>[2x]PKIVVVGAVAGGATCASQIRRLDKESDIIIFEKDRDMSFANCALPYVIGEVVEDRRYALAYTPEKFYDRKQITVKTYHEVIAINDERQTVSVLNRKTNEQFEESYDKLILSPGASANSLGFESDITFTLRNLEDTDAIDQFIKANQVDKVLVVGAGYVSLEVLENLYERGLHPTLIHRSDKINKLMDADMNQPILDELDKREIPYRLNEEINAINGNEITF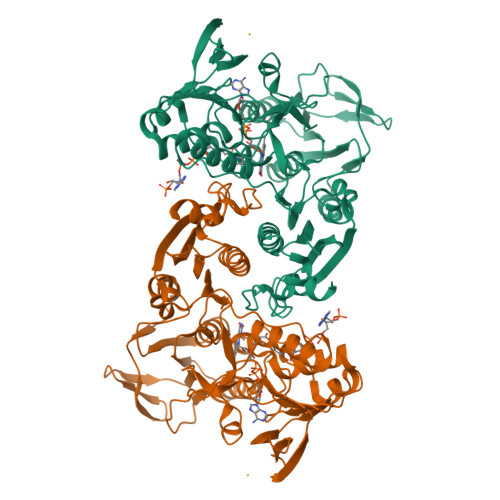KSGKVEHYDMIIEGVGTHPNSKFIESSNIKLDRKGFIPVNDKFETNVPNIYAIGDIATSHYRHVDLPASVPLAWGAHRAASIVAEQIAGNDTIEFKGFLGNNIVKFFDYTFASVGVKPNELKQFDYKMVEVTQGAHANYYPGNSPLHLRVYYDTSNRQILRAAAVGKEGADKRIDVLSMAMMNQLTVDELTEFEVAYAPPYSHPKDLINMIGYKA>[4x]MKMDKKTIVWFRRDLRIEDNPALAAAAHEGSVFPVFIWCPEEEGQFYPGRASRWWMKQSLAHLSQSLKALGSDLTLIKTHNTISAILDCIRVTGATKVVFNHLYDPVSLVRDHTVKEKLVERGISVQSYNGDLLYEPWEIYCEKGKPFTSFNSYWKKCLDMSIESVMLPPPWRLMPITAAAEAIWACSIEELGLENEAEKPSNALLTRAWSPGWSNADKLLNEFIEKQLIDYAKNSKKVVGNSTSLLSPYLHFGEISVRHVFQCARMKQIIWARDKNSEGEESADLFLRGIGLREYSRYICFNFPFTHEQSLLSHLRFFPWDADVDKFKAWRQGRTGYPLVDAGMRELWATGWMHNRIRVIVSSFAVKFLLLPAKWGMKYFWDTLLDADLECDILGWQYISGSIPDGHELDRLDNPALQGAKYDPEGEYIRQWLP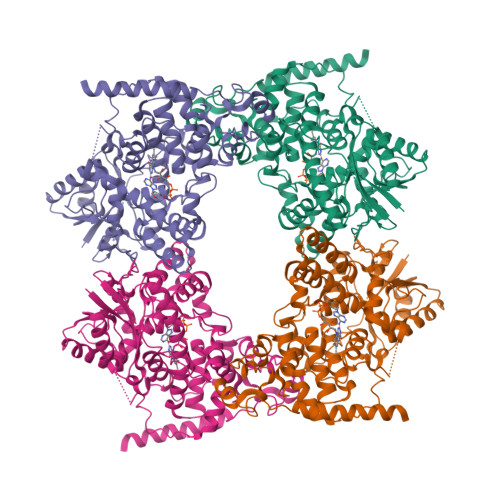ELARLPTEWIHHPWDAPLTVLKASGVELGTNYAKPIVDIDTARELLAKAISRTREAQIMIGAAPDEIVADSFEALGANTIKEPGLCPSVSSNDQQVPSAVRYNGSKRVKPEEEEERDMKKSRGFDERELFSTAESSSSSSVFFVSQSCSLASEGKNLEGIQDSSDQITTSLGKNGCK MazEF is a TA system implicated in the formation of “persisters cells” of M. tb, which contain more than 10 such members. All the MazF toxins from the family are RNases, capable of cleaving various types of RNA including mRNA, tRNA, or rRNA. To better reflect the specificity of MazF-mt3 in M. tb, the so-called MORE RNA-seq was developed, which identified the cleavage sequence as U↓CCUU. Here we report crystal structures of MazF-mt3 in its apo form and in complex with the C-terminal half of MazE-mt3.

Through extensive trials, only the MazE-mt346−82 peptide produced suitable crystals for structure determination. The final model contained three toxin monomers (chains A, B, and C) and two antitoxin monomers (chains D and I) with a space group P3121. These molecules formed peculiar combinations: while the toxin dimer comprising chains A/B complexed with one of the antitoxins (chain I) in a stoichiometry of 2:1 (named “the complete complex” hereinafter), the remaining toxin (chain C) associated with the other antitoxin (chain D) in a stoichiometry of 1:1 (“the half complex”). The β1–β2 loops of the three toxin molecules were still disordered while chains I and D resolved residues Leu46-Thr77 and Thr47-Ala69 of the antitoxins, respectively. The binding of the peptide did not change the structure of the toxin dimer, which is common among the MazEF members. The peptide formed two short helices (α3-α4) situated across the deep crevice formed by the dimer, and the α4-helix was located in the proximity to the loops. The total buried surface is 2392.8 Å2 between the MazF-mt3 dimer and its contacting MazE-mt3 monomer. Taken together, most intermolecular contacts are from the α3-helix and the α3-α4 loop. In contrast, the last helix (α4, fragment Thr60-Trp82) or the second-to-last helix (α3, fragment Leu46-Gly59) of the antitoxin exhibited minimal inhibitory effects. It was the peptide corresponding to the last two helices (α3-α4, i.e., Leu46-Trp82) with a molar ratio of 1:4 (antitoxin/toxin) that reduced the cleavage of the enzyme by 15%. MazF-mt3 represents scenario 3, where the cross-subunit loops remain open upon the binding of MazE-mt3.

>GPELMVISRAEIYWADLGPPSGSQPAKRRPVLVIQSDPYNASRLATVIAAVITSNTALAAMPGNVFLPATTTRLPRDSVVNVTAIVTLNKTDLTDRVGEVPASLMHEVDRGLRRVLDL[3x];>[2x]LTGQIDRALESIHGTDEAEALAVANAYRVLETMDDEW> MERLFEELAGEAVKELLRAVRGTFFCRSTAERLRRNVEPLLPLVQPQAAQGGGGWGHGRSAGELAELAAQLREALELARRAASAPRW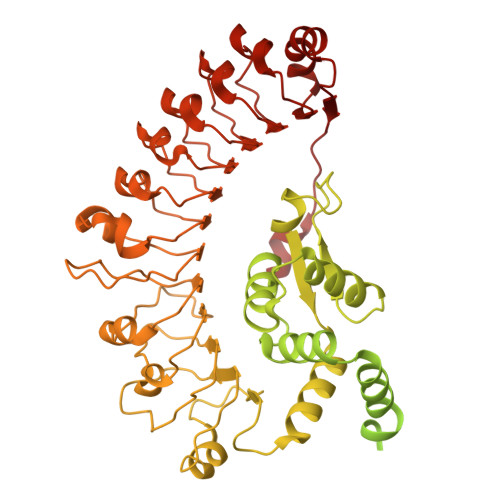NVYRTAQLARRMEAADTAIARWLSRHAPAHVLDGVRRLRDEADARIGRLERRVEEVAAAQQQQQAAATALPPPAISLPFALPPPPPPPKAMAMMAMDTPPTKGMAVGMEVELPFPDDEEDESMVGGGVRVGKEKVKEMVMSGGGGGWEAVGICGMGGSGKTTLAMEIFKDHKIRGYFSDRVFFETISQSANLDTIKMKLWEQISGNLVLGAYNQIPEWQLKLGPRDKGPVLVILDDVWSLSQLEELIFKFPGCKTLVVSRFKFPSLVTRTYEMELLDEEAALSVFCRAAFDQESVPRTADKKLVRQVAAECRGLPLALKVIGASLRDQPPKIWLSAKNRLSRGETISDSHETKLLERMAASIECLSGKVRECFLDLGCFPEDKKIPLDVLINIWMEIHDLDEPDAFAILVELSNKNLLTLVNDAQNKAGDLYSSYHDFSVTQHDVLRDLALHMSGRDALNNRRRLVMPRREESLPKDWQRNKDTPFEAQIVSIHTGEMKESDWFQMSFPKAEVLILNFASSVYYLPPFIATMQNLKALVLINYGTISATLDNLSAFTTLSDLRSLWLEKITLPPLPKTTIPLKNLRKISLVLCELTNSLRGSKVDLSMTFPRLSNLTIDHCIDLKELPSSICEISSLESISISNCHDLTELPYELGKLHCLSILRVYACPALWRLPPSVCSLKRLKYLDISQCVNLTDLPEELGHLTSLEKIDMRECSRLRSLPRSSSSLKSLGHVVCDEETALLWREAEQVIPDLRVQVAEECYNLDWLVD>MHHHHHHTSKIEQPRWASKDDAAGKASTPDEKI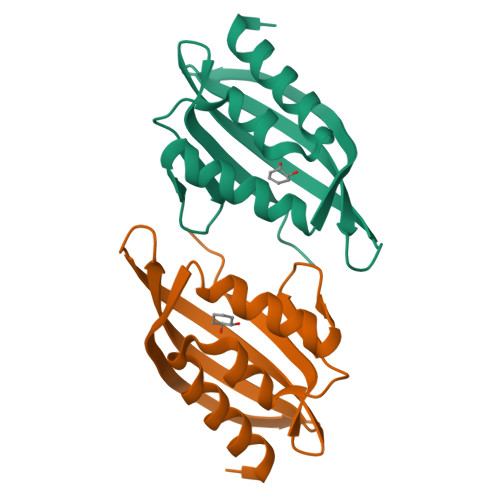VLEFMDALTSNDAAKLIDYFAEDTMYQNMPLPPAYGRDAVEQTLAGFFKVFSIDAVETFHIGSTKGLVYTERVDVLRALPTGKSYNVSVLGVFQLTEGKITGWRDYFDLREVEEAVDLPFRG[2x]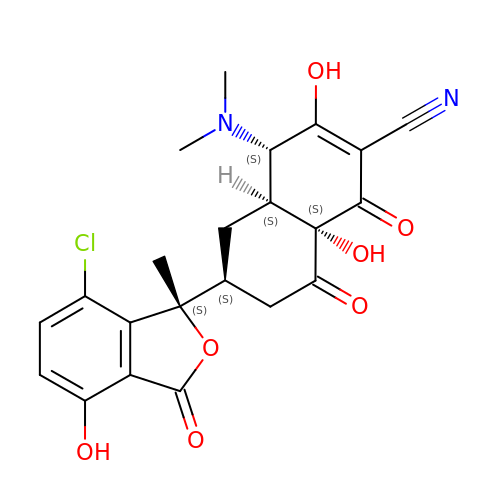(4S,4AS,6S,8AS)-6-[(1S)-7-CHLORO-4-HYDROXY-1-METHYL-3-OXO-1,3-DIHYDRO-2-BENZOFURAN-1-YL]-4-(DIMETHYLAMINO)-3,8A-DIHYDROXY-1,8-DIOXO-1,4,4A,5,6,7,8,8A-OCTAHYDRONAPHTHALENE-2-CARBONITRILE | C22 H21 Cl N2 O7 | LLGMOYSDYFLOGF-REEKZYMCSA-N> MHLLVRPEPFADEALESYFLRLSQENGFERYRIF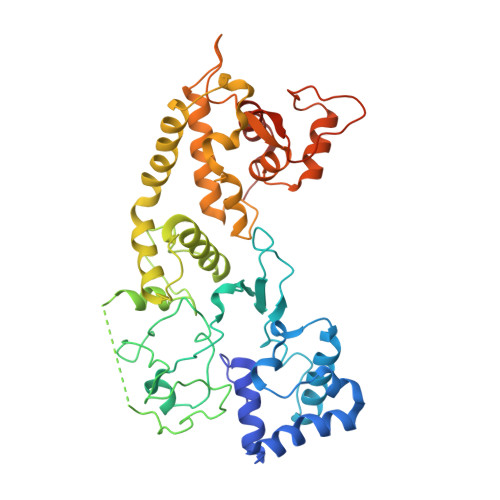SGSVQDWLHTTDHAAAGAFPLELSRLNIFHASRSSGLRVRALQLVDRLTDGAPFRLLQLALCHSAISFGNHYKAVHRSGVDIPLSFIRVHQIPCCPDCLRESAYVRQCWHFKPYVGCHRHGGRLIYSCPACGESLNYLASESINHCQCGFDLRTASTVPAQPDEIQLSALAYGCSFESSNPLLAIGSLSARFGALYWYQQRYLSDHEAVRDDRALTKAIGHFTAWPDAFWRELQQMVDDALVRQTKPLNHTDFVDVFGSVVADCRQIPMRNTGQNFILKNLIGFLTDLVARHPQCRVANVGDLLLSAVDAATLLSTSVEQVRRLHHEGFLPLSIRPASRNTVSPHRAVFHLRHVVELRQARMQSHHDHSSTYLPAW(1~{R})-2-ethanoyl-~{N}-[4-[1,1,1,3,3,3-hexakis(fluoranyl)-2-oxidanyl-propan-2-yl]phenyl]-5-methylsulfonyl-1,3-dihydroisoindole-1-carboxamide 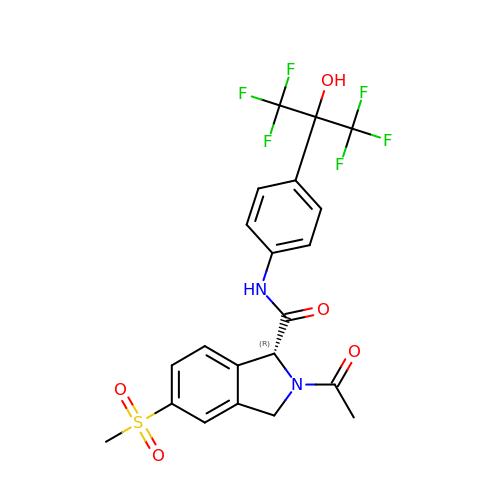| C21 H18 F6 N2 O5 S | QYYZXEPEVBXNNA-QGZVFWFLSA-N>MALDKLDLYVIITLVVAVAAYFAKNQFLDQPQDTGFLNTDSGSNSRDVLSTLKKNNKNTLLLFGSQTGTAEDYANKLSRELHSRFGLKTMVADFADYDWDNFGDITEDILVFFIVATYGEGEPTDNADEFHTWLTEEADTLSTLRYTVFGLGNSTYEFFNAIGRKFDRLLSEKGGDRFAEYAEGDDGTGTLDEDFMAWKDNVFDALKNDLNFEEKELKYEPNVKLTERDDLSAADSQVSLGEPNKKYINSEGIDLTKGPFDHTHPYLARITETRELFS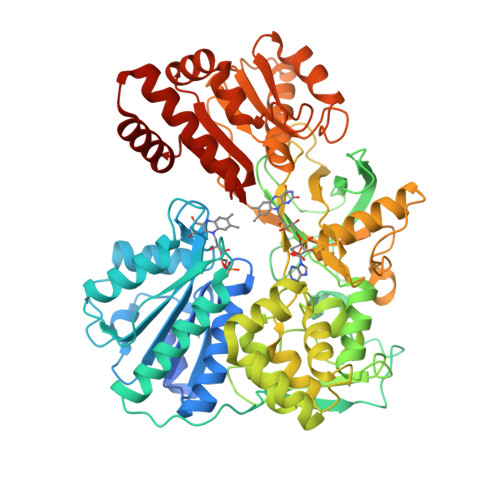SKERHCIHVEFDISESNLKYTTGDHLAIWPSNSDENIKQFAKCFGLEDKLDTVIELKALDSTYTIPFPTPITYGAVIRHHLEISGPVSRQFFLSIAGFAPDEETKKTFTRLGGDKQEFATKVTRRKFNIADALLYSSNNTPWSDVPFEFLIENIQHLTPRYYSISSSSLSEKQLINVTAVVEAEEEADGRPVTGVVTNLLKNIEIAQNKTGEKPLVHYDLSGPRGKFNKFKLPVHVRRSNFKLPKNSTTPVILIGPGTGVAPLRGFVRERVQQVKNGVNVGKTLLFYGCRNSNEDFLYKQEWAEYASVLGENFEMFNAFSRQDPSKKVYVQDKILENSQLVHELLTEGAIIYVCGDASRMARDVQTTISKIVAKSREISEDKAAELVKSWKVQNRYQEDVW[2x]>GMEDYSREYSEVLLQLKELQDSEAFLEPVNWKKLGLDDY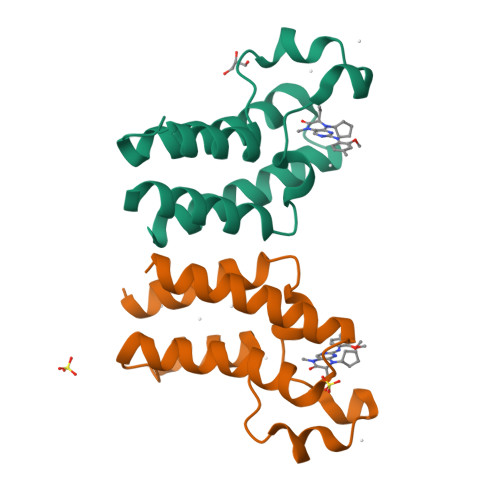PDIVKNPMDLKTIGKKIKANFYTKAEQFWADIDLIWHNCQLYNHESSEVYQQSIRMQDAANNLRDML[2x]> MAGSSFSGKYQLQSQ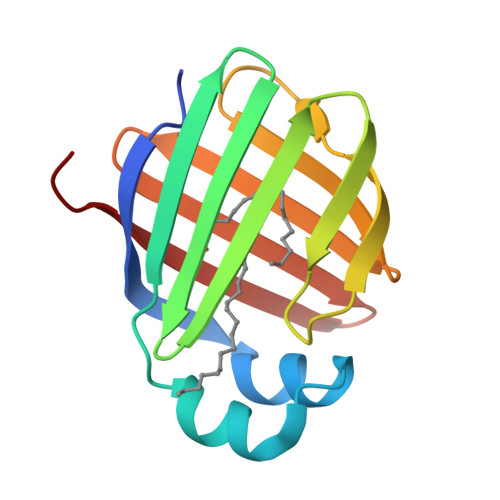ENFEAFMKAIGLPEELIQKGKDIKGVSEIVQNGKHFKFTITAGSKVIQNEFTVGEECELETMTGEKVKTVVQLEGDNKLVTTFKNIKSVTELNGDIITNTMTLGDIVFKRISKRIGT>RRELKLLLLGTGESGKSTFIKQMRIIHGSGYSDEDKRGFTKLVYQNIFTAMQAMIRAMDTLKIPYKYEHNKAHAQLVREVDVEKVSAFENPYVDAIKSLWNDPGIQECYDRRREYQLSDSTKYYLNDLDRVADPSYLPTQQDVLRVRVPTTGIIEYPFDLQSVIFRMVDVGGQRSERRKWIHCFENVTSIMFLVALSEYDQVLVESDNENRMEESKALFRTIITYPWFQNSSVILFLNKKDLLEEKIMYSHLVDYFPEYDGPQRDAQAAREFILKMFVDLNPDSDKIIYSHFTCATDTENIRFVFAAVKDTILQ[3x];>[3x]SMLKRLSTEEATRWADSFDVLLSHKYGVAAFRAFLKTEFSEENLEFWLACEEFKKTRSTAKLVSKAHRIFE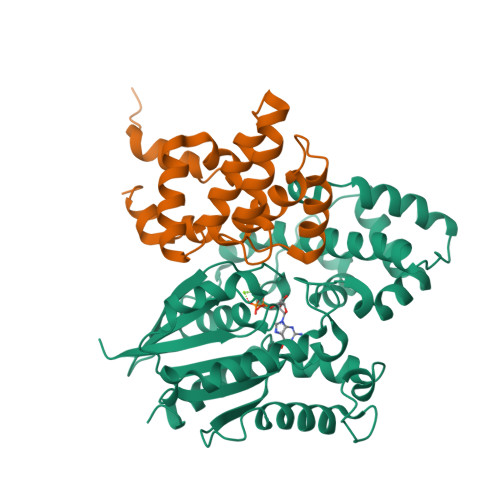EFVDVQAPREVNIDFQTREATRKNLQEPSLTCFDQAQGKVHSLMEKDSYPRFLRSKMYLDLLS> GSHMTDNLPDRSSVTNNMARVELPVINITSFGTKPSFLNIQKSASTKSLNLIAENSGDTETKEFESSESVVLNHLNRYVFPGSLLMGNSIQDLNYKPVFASLNPITVSLSIPAINQNTAITITNPSLSATRAAVYNYLKTADFTQNGQLSYSIQQFSSYDELKVAFGSNVNSRNLFGKNSSSTNVEEGMVARQSGFYVKFYQTSFTLDMDVPNGSLVKDNNFDSEGIEPVYVSSISYGRMGILAIETNEKAEDAKRIINETFNKLFYKKQTNFSQEEKSFIEGADFNLYLVGGDGSTASQSFKGYEAFVNHVSQGTFSKDQPGVPIFCSYSYLKDNSPVKTKFKFDIKRPPLYVKLVKENMKDINFNDPDGGIYDNKKEAILKIYFYKNRSLVPTLPNPYINFKIREKKKKWQSIAPVYYSSLDQVPFNISERILTKQNTLQNIFATIQTQDNTEFSLISRIIRGGGRQNPVPAGFRAIEINDYELVEDSNYII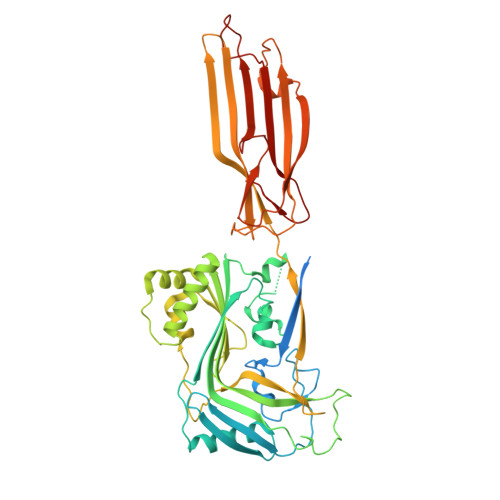IKD>GMIPIVDSRIGAYLDGLLPEADPVVAAMEQIARERNIPIVDRQTGRLLYLLARIKQPQLVVVPGDGLGCASWWFARAISISSRVVMIDPDRDNVEHARRMLHDNGLIDRVELQVGDPLGIAAGQRDIDILFMDCDVFNGADVLERMNRCLAKNALLIAVNALRRGSVAESHEDPETAALREF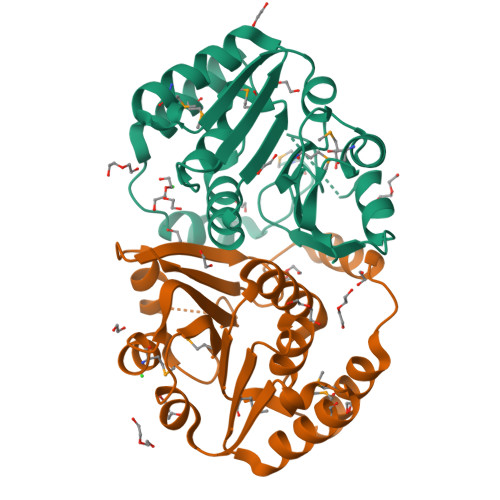NHHLSRRRDFFTTIVPVGNGVLLGYRLS[3x]6,9-dimethyl[1,3]dioxolo[4,5-h]quinolin-8(9H)-one 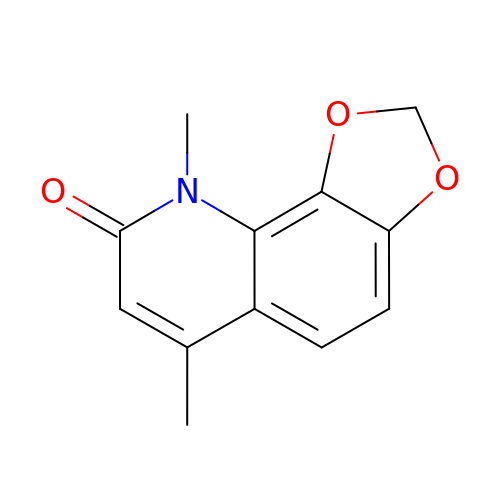| C12 H11 N O3 | FEMZVADPTYXZIF-UHFFFAOYSA-N> TDFNQKIE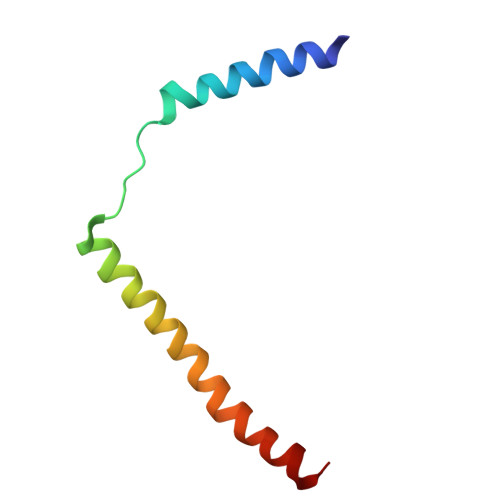QLKEFIEECRRVWLVLKKPTKDEYLAVAKVTALGISLLGIIGYIIHVPATYIKGILK> MEAEQVWKLWRRVLRDERLQAQLFSATDATHWLSGFSESESKILSVYAQQFDRVKWFVENYQFRLVNSFLNALETGAPLSLRALLHINVDLNAQSKAFLRDRQWRDYGPQVYTYCEDVLGFLAEADELQGYPEILDLMRLERESVRLYRGLVDPESLPADNRYQRTSMARLYETRFALSGWLRQKDQLGLTRLPESTEHVLIYLPTLQARHKFTLINAQAARLYNCLEQPQSAAGLFMLINSDSASVPGSADLALL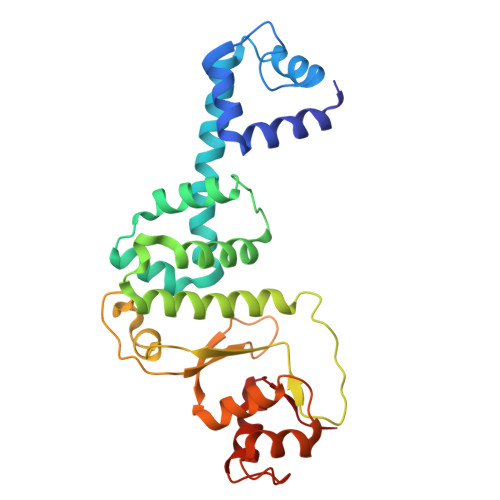DRLEQLNAIRKPL> DCGQPRNLPNGDFRYTTTMGVNTYKARIQYYCHEPYYKMQTRAGSRESEQGVYTCTAQGIWKNEQKGEK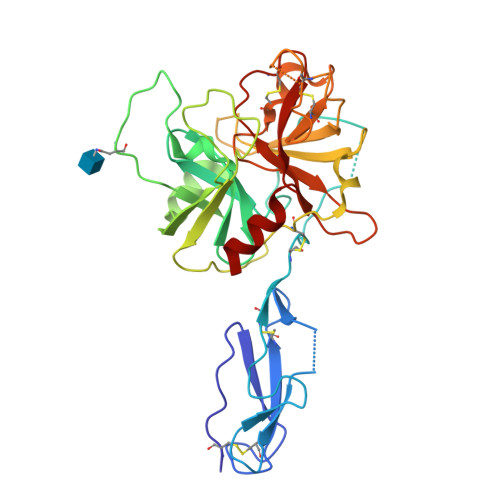IPRCLPVCGKPVNPVEQRQRIIGGQKAKMGNFPWQVFTNIHGRGGGALLGDRWILTAAHTLYPKEHEAQSNASLDVFLGHTNVEELMKLGNHPIRRVSVHPDYRQDESYNFEGDIALLELENSVTLGPNLLPICLPDNDTFYDLGLMGYVSGFGVMEEKIAHDLRFVRLPVANPQACENWLRGKNRMDVFSQNMFCAGHPSLKQDACQGDAGGVFAVRDPNTDRWVATGIVSWGIGCSRGYGFYTKVLNYVDWIKKEME> LPTSNPAQELEARQLGRTTRDDLINGNSASCRDVIFIYAR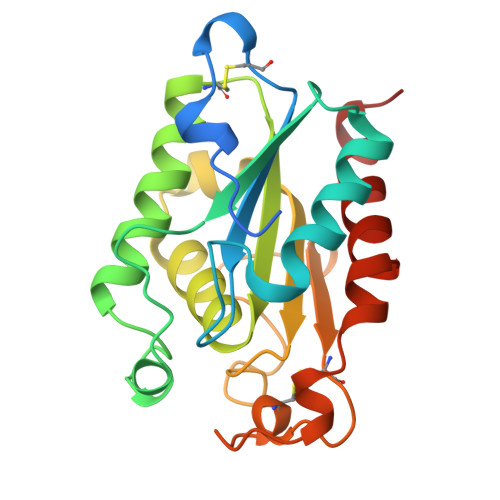GSTETGNLGTLGPSIASNLESAFGKDGVWIQGVGGAYRATLGDAALPRGTSSAAIREMLGLFQQANTKCPDATLIAGGYSQGAALAAASIEDLDSAIRDKIAGTVLFGYTKNLQNRGRIPNYPADRTKVFCNTGDLVCTGSLIVAAPHLAYGPDARGPAPEFLIEKVRAVRGSA>[2x]SFISDGVFESQSLVLGRNLLQTKKTCPVNFEFMNYTIITSKCKGPKYPPKECCGAFKDFACPYTDQLN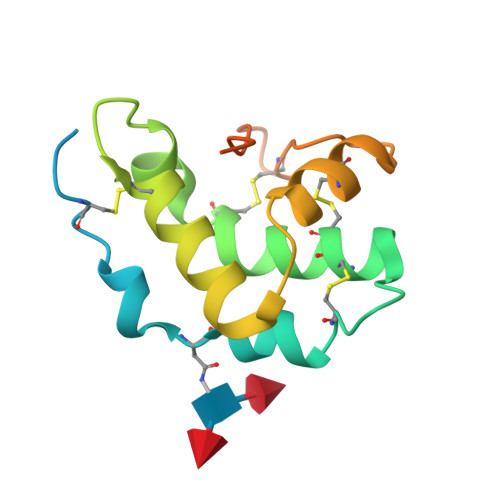DLSSDCATTMFSYINLYGKYPPGLFANQCKEGKEGLECPAGSQLPPETSAEVNAATTSSSRLWLTVSA1-[3-tert-butyl-1-(4-methylphenyl)-1H-pyrazol-5-yl]-3-(2-hydroxyethyl)urea 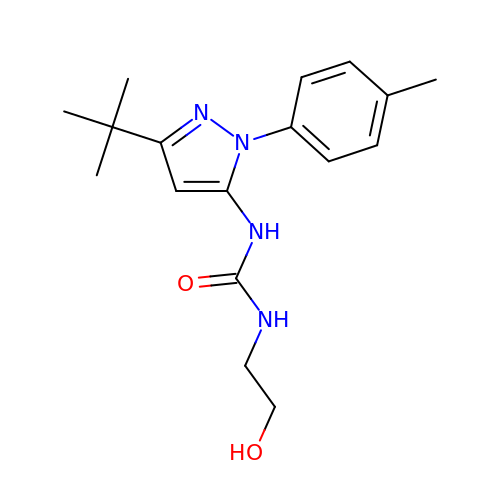| C17 H24 N4 O2 | QTPQATQIABNKIE-UHFFFAOYSA-N N-[(1R)-1-[(BENZYLSULFONYL)METHYL]-2-{[(1S)-1-METHYL-2-{[4-(TRIFLUOROMETHOXY)PHENYL]AMINO}ETHYL]AMINO}-2-OXOETHYL]MORPHOLINE-4-CARBOXAMIDE | C25 H31 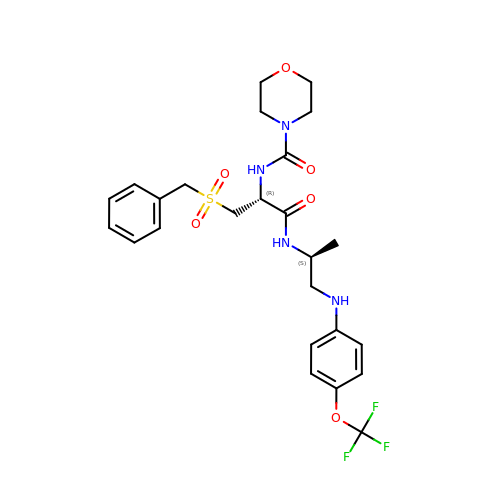F3 N4 O6 S | LIOLGHUQUQDMDF-AVRDEDQJSA-N[(2R,3S,4R,5R)-5-(6-amino-9H-purin-9-yl)-3,4-dihydroxytetrahydrofuran-2-yl]methyl [(2R,3R,4S)-4-fluoro-3-hydroxytetrahydrofuran-2-yl]methyl dihydrogen diphosphate | C15 H22 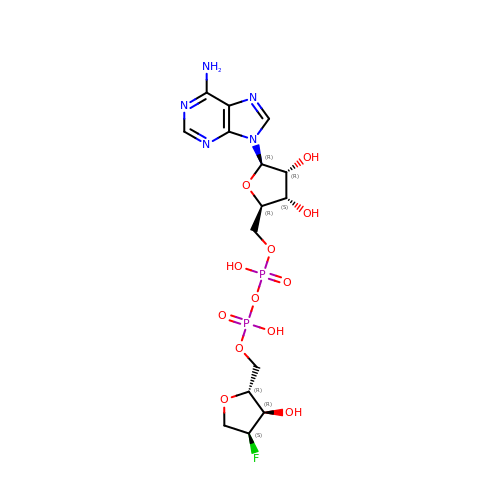F N5 O12 P2 | GOCJJDZHXMDJEZ-AOOZFPJJSA-N>MRIVEIREQTAGIKSDIANAFIDFSQMTCSVVAVVTDVVRDGKPVIGYGFNSNGRYAAGGLLRERFIPRLMSAAPDSLLDETGENLDPFRIWTRLMTNEKPGGHGERSVAVGTIDMAVWDAVAKIAGVPLYRLLADRFRGGVADDGVWVYAAGGYYYPGKDVKALQDEMRSYRDRGYRVVKMKIGGAPLAEDLRRIDAVLEVVGSGDNLCVDANGRFDIDTAIAYGEALKPYGLFWYEEAGDPLDYALQAELAKHY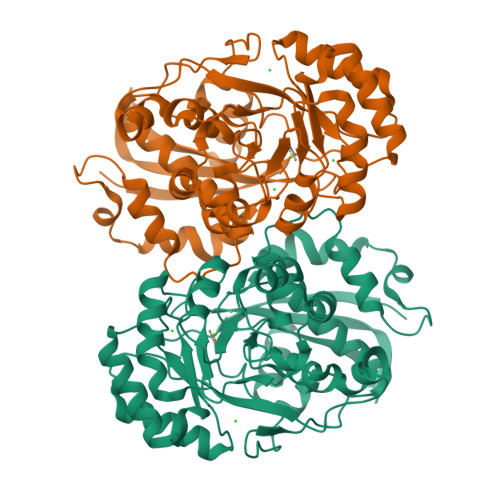DRPMATGENLFSHQDARNLIRHGGMRPDRDWLQFDCALSYGLVEYLRTLDMLKENGWSSRRVVPHGGHQMSLNIAAGLHLGGNESYPDVFKPFCGFADGIAVEDGRVRLPDLPGVGFEAKSELFATMSGLLGTR[2x]(1~{R},2~{S})-2-[[(6-bromanyl-1~{H}-indazol-4-yl)amino]methyl]cyclohexan-1-ol 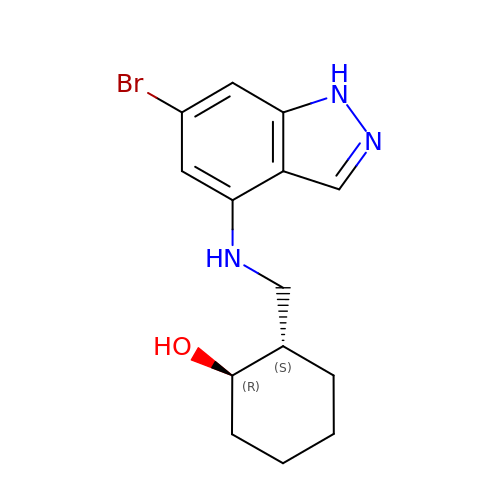| C14 H18 Br N3 O | KBSUKSFOQICUON-LKFCYVNXSA-N>NMDWALFLTFLAACGAPATTGALLKPDEWYDNLNKPWWNPPRWVFPLAWTSLYFLMSLAAMRVAQLEGSGQALAFYAAQLAFNTLWTPVFFGMKRMATALAVVMVMWLFVAATMWAFFQLDTWAGVLFVPYLIWATATTGLNFEAMRLNWNRP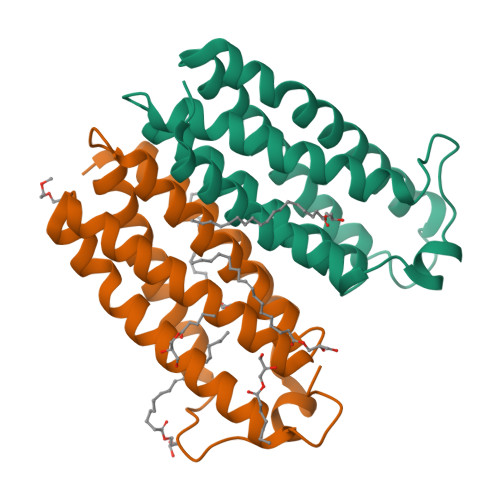EAR[2x]>PNFSGNWKIIRSENFEELLKVLGVNVMLRKIAVAAASK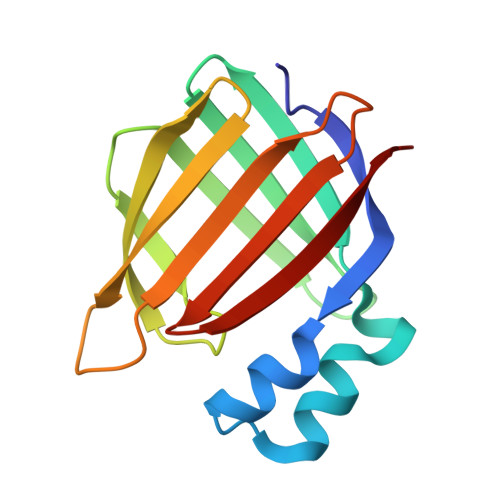PAVEIKQEGDTFYIKTSTTVRTTEINFKVGEEFEEQTVDGRPCKSLVKWESENKMVCEQKLLKGEGPKTSWTLELTNDGELIETMTADDVVCTKVFVRE[2x]(3S,4R)-2-(4-AMINO-5H-PYRROLO[3,2-D]PYRIMIDIN-7-YL)-5-[(METHYLSULFANYL)METHYL]PYRROLIDINE-3,4-DIOL 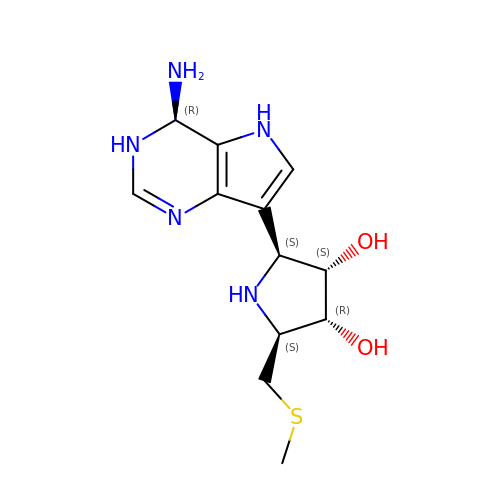| C12 H19 N5 O2 S | YLCQGEBEQIBOOJ-BOFBLULFSA-N>MKYKEPFGVKLDFETGIIENAKKSVRRLSDMKGYFIDEEAWKKMVEEGDPVVYEVYAIEQEEKEGDLNFATTVLYPGKVGNEFFMTKGHYHSKIDRAEVYFALKGKGGMLLQTPEGEARFIEMEPGTIVYVPPYWAHRTINTGDKPFIFLALYPADAGHDYGTIAEKG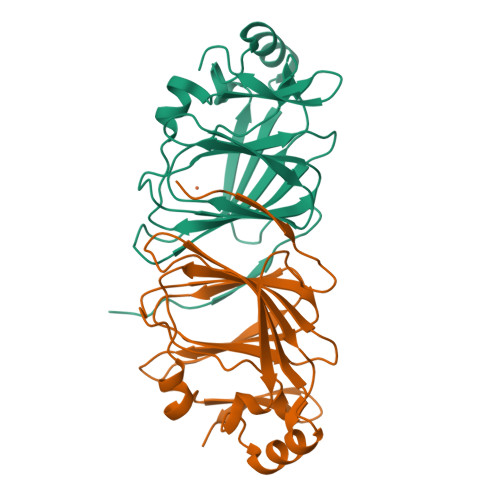FSKIVVEENGKVVVKDNPKWRM[2x]> MDTEKLMKAGEIAKKVREKAIKLARPGMLLLELAESIEKMIMELGGKPAFPVGLSINEIAAHYTPYKGDTTVLKEGDYLKIDVG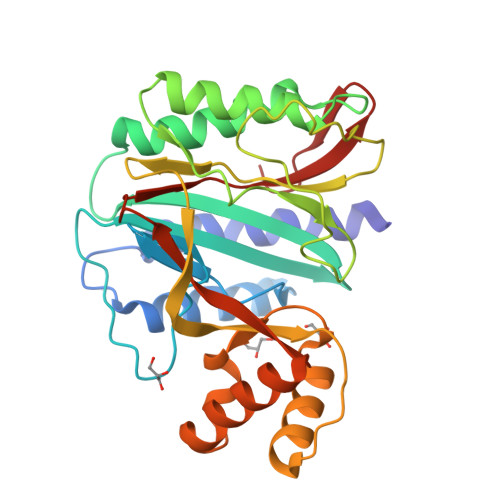VHIDGFIADTAVTVRVGMEEDELMEAAKEALNAAISVARAGVEIKELGKAIENEIRKRGFKPIVNLSGHKIERYKLHAGISIPNIYRPHDNYVLKEGDVFAIEPFATIGAGQVIEVPPTLIYMYVRDVPVRVAQARFLLAKIKREYGTLPFAYRWLQNDMPEGQLKLALKTLEKAGAIYGYPVLKEIRNGIVAQFEHTIIVEKDSVIVTTE>MDVSFRLSGATTTSYGVFIKNLREALPYERKVYNIPLLRSSISGSGRYTLLHLTNYADETISVAVDVTNVYIMGYLAGDVSYFFNEASATEAAKFVFKDAKKKVTLPYSGNYERLQTAAGKIRENIPLGLPALDSAITTLYY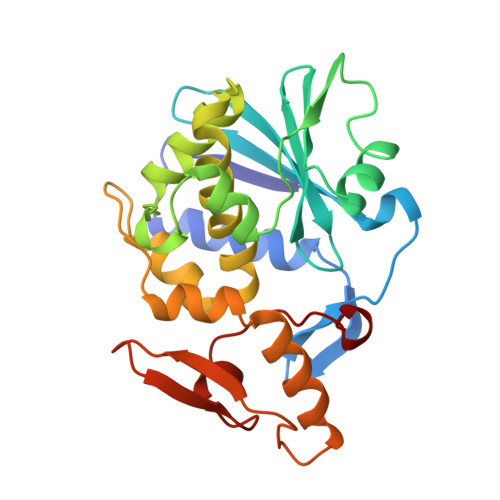YTASSAASALLVLIQSTAESARYKFIEQQIGKRVDKTFLPSLATISLENNWSALSKQIQIASTNNGQFESPVVLIDGNNQRVSITNASARVVTSNIALLLNRNNIA[2x]> AMGQSTSNHLWLLSDILGQGATANVFRGRHKKTGDLFAIKVFNNISFLRPVDVQMREFEVLKKLNHKNIVKLFAIEEETTTRHKVLIMEFCPCGSLYTVLEEPSNAYGLPESEFLIVLRDVVGGMNHLRENGIVHRDIKPGNIMRVIGEDGQSVYKLTDFGAARELEDDEQFVALYGTEEYLHPDMYERAVLRKDHQKKYGATVDLWSIGVTFYHAATGSLPFRPFEGPRRNKEVMYKIITGKPSGAISGVQKAENGPIDWSGDMPVSCSLSRGLQVLLTPVLANILEADQEKCWGFDQFFAETSDILHRMVIHVFSLQQMTAHKIYIHSYNTATIFHELVYKQTKIISSNQELIYEGRRLVLEPGRLAQHFPKTTEENPIFVVSREPLNTIGLIYEKISLPKVHPRYDLDGDASMAKAITGVVCYACRIASTLLLYQELMRKGIRWLIELIKDDYNETVHKKTEVVI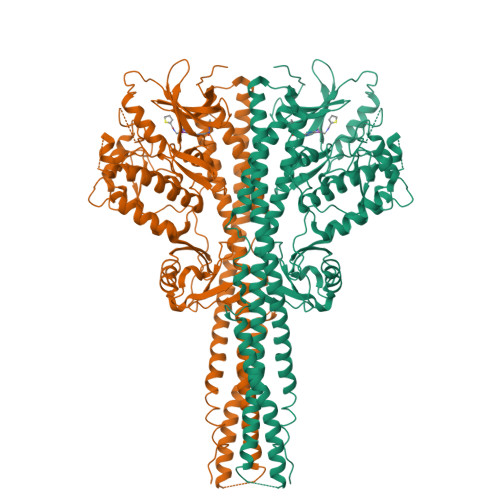TLDFCIRNIEKTVKVYEKLMKINLEAAELGEISDIHTKLLRLSSSQGTIETSLQDIDSRLSPGGSLADAWAHQEGTHPKDRNVEKLQVLLNCMTEIYYQFKKDKAERRLAYNEEQIHKFDKQKLYYHATKAMTHFTDECVKKYEAFLNKSEEWIRKMLHLRKQLLSLTNQCFDIEEEVSKYQEYTNELQET> MNSIKFPILDRTTKNSVISTTLNDLSNWSRLSSLWPLLYGTSCCFIEFASLIGSRFDFDRYGLVPRSSPRQADLILTAGTVTMKMAPSLVRLYEQMPEPKYVIAMGACTITGGMFSTDSYSTVRGVDKLIPVDVYLPGCPPKPEAVIDAITKLRKKIAREIYKDRIRPQQGNRC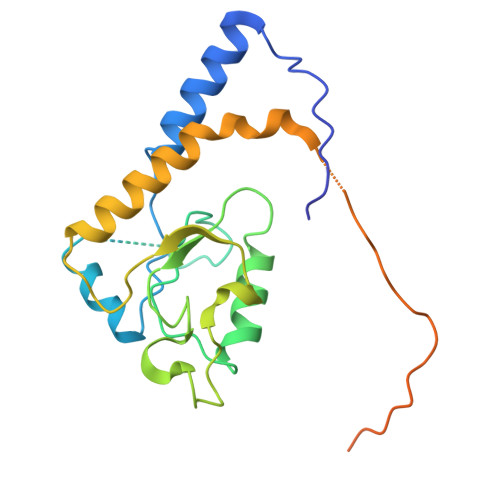FTTNHKFFVVRSPHIGNYDQELLYPPSSTSEISTETFFKYKSPVSSHELVN> RKLCSLDNGDCDQFCHEEQNSVVCSCARGYTLADNGKACIPTGPYPCGKQTL;> F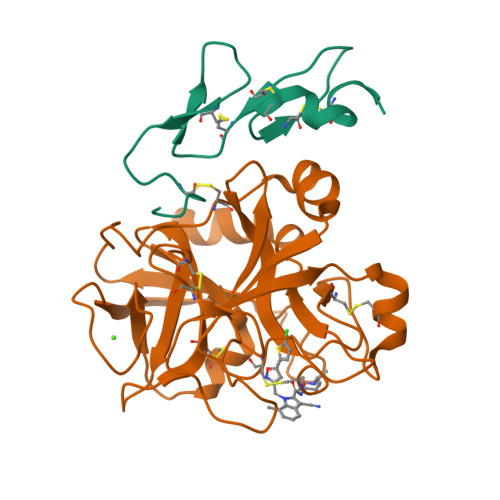NQTQPERGDNNLTRIVGGQECKDGECPWQALLINEENEGFCGGTILSEFYILTAAHCLYQAKRFKVRVGDRNTEQEEGGEAVHEVEVVIKHNRFTKETYDFDIAVLRLKTPITFRMNVAPACLPERDWAESTLMTQKTGIVSGFGRTHEKGRQSTRLKMLEVPYVDRNSCKLSSSFIITQNMFCAGYDTKQEDACQGDSGGPHVTRFKDTYFVTGIVSWGEGCARKGKYGIYTKVTAFLKWIDRSMKT N-[4-(piperidin-1-ylsulfonyl)benzyl]-1H-pyrrolo[3,2-c]pyridine-2-carboxamide | C20 H22 N4 O3 S | 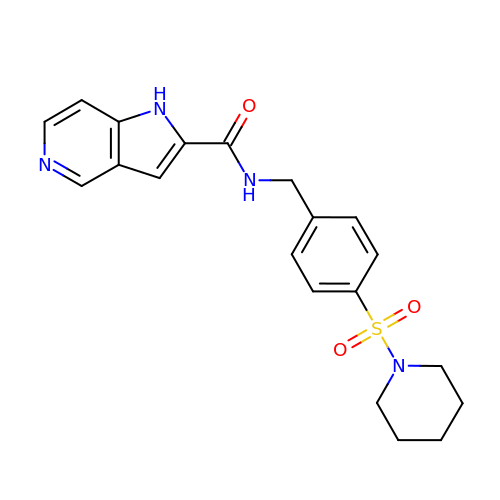AOQJDTPGTHTUAQ-UHFFFAOYSA-N> MVEKEEAGGGISEEEAAQYDRQIRLWGLEAQKRLRASRVLLVGLKGLGAEIAKNLILAGVKGLTMLDHEQVTPED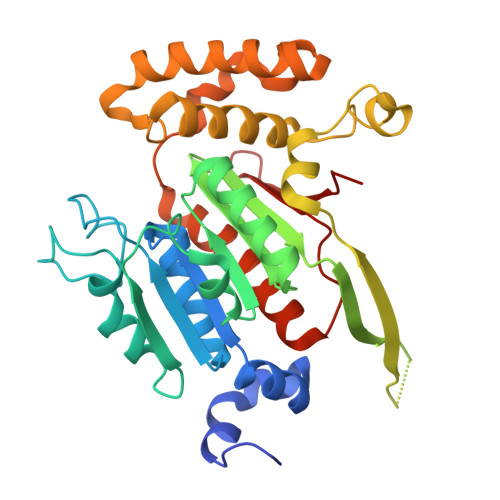PGAQFLIRTGSVGRNRAEASLERAQNLNPMVDVKVDTEDIEKKPESFFTQFDAVCLTCCSRDVIVKVDQICHKNSIKFFTGDVFGYHGYTFANLGEHEFVEEKTKVAKVSQGVEDGPDTKRAKLDSSETTMVKKKVVFCPVKEALEVDWSSEKAKAALKRTTSDYFLLQVLLKFRTDKGRDPSSDTYEEDSELLLQIRNDVLDSLGISPDLLPEDFVRYCFSEMAPVCAVVGGILAQEIVKALSQRDPPHNNFFFFDGMKGNGIVECLGPK(1R)-1-[((1E)-{3-HYDROXY-2-METHYL-5-[(PHOSPHONOOXY)METHYL]PYRIDIN-4-YL}METHYLENE)AMINO]-1-PHENYLETHYLPHOSPHONIC 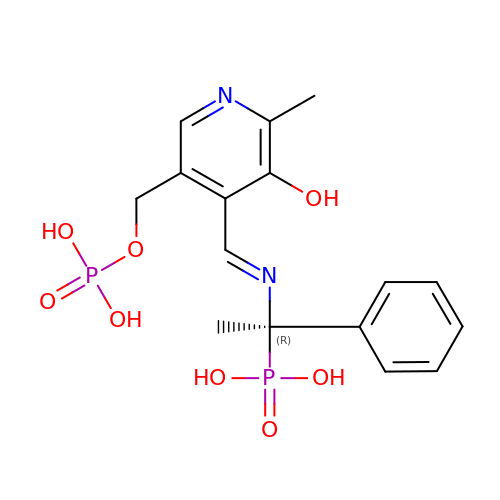ACID | C16 H20 N2 O8 P2 | YMGMBGLRDKSMMV-TWIVVOHQSA-N[2-(4-cyclopentylpyridin-3-yl)-1,3-benzoxazol-6-yl]-[6-(3-cyclopropyl-1,2,4-triazol-1-yl)-2-azaspiro[3.3]heptan-2-yl]methanone 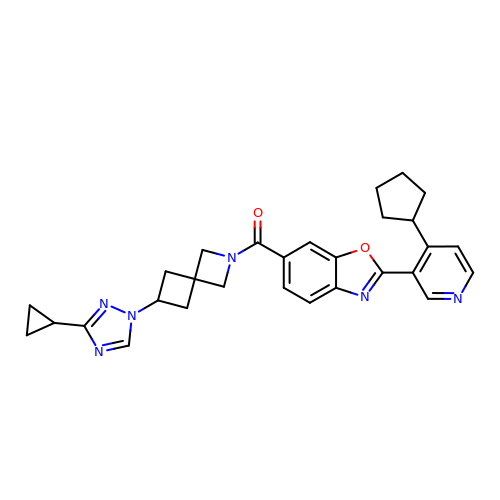| C29 H30 N6 O2 | NRSBFRBTSIBXDY-UHFFFAOYSA-N>[2x]MAHHHHHHMHEIVDKNGKKVQKNNLNDEIKIIFTALDGTLLNSENKVSEQNLESLIRAQEKGIKVVIATGRSIFSVENVIGEHVKKNRISLLPGIY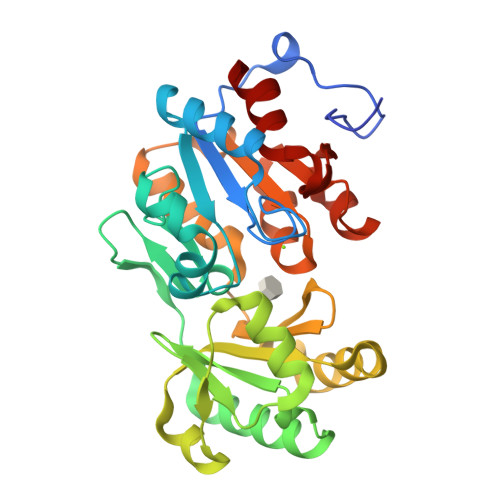MNGCVTFDEKGSRVIDRIMNNDLKMEIHEFSKQINISKYAIWFCLEKTYCFEINDCIREYMEVEALNPDVIEDNMLEGLTVYKVLFSLPENILENTLKLCREKFSHRINVANTFQSYVELFHQHTNKFEGVKEICKYYNISLNNALAMGDGENDIEMLSGLTHSVGVHNASEKVKNSAAYVGPSNNEHAISHVLKTFCDI> NIPFTNNLLFSGQVLYGDGRLTAKSHQLVMQGDCNLVLYGGKYGW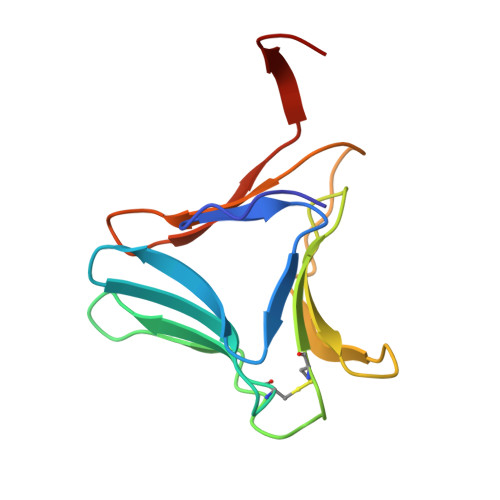QSNTHGNGEHCFLRLNHKGELIIKDDDFKTIWSSSSSSKHGDYVLILRDDGFAVIYGPAIWETSPQ> GCVSIIGRLHVNQRGSGSASITAYAQQTRGLLGAIVVSMTGRDRTEQAGEVQILSTVSQSFLGTTISGVLWTVYHGAGNKTLAGLRGPVTQMYSSAEGDLVGWPSPPGTKSLEPCKCGAVDLYLVTRNADVIPARRRGDKRGALLSPRPISTLKGSSGGPVLCPRGHVVGLFRAAVCSRGVAKSIDFIPVETLDVVTRSPTFSDNSTPPAVPQTYQVGYLHAPTGSGKSTKVPVAYAAQGYKVLVLNPSVAATLGFGAYLSKAHGINPNIRT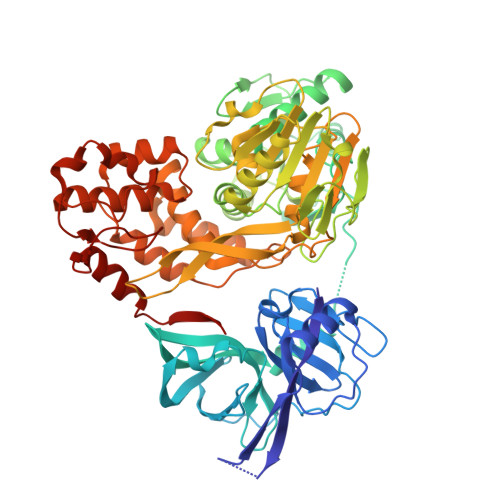GVRTVMTGEAITYSTYGKFLADGGCASGAYDIIICDECHAVDATSILGIGTVLDQAETAGVRLTVLATATPPGSVTTPHPDIEEVGLGREGEIPFYGRAIPLSCIKGGRHLIFCHSKKKCDELAAALRGMGLNAVAYYRGLDVSIIPAQGDVVVVATDALMTGYTGDFDSVIDCNVAVTQAVDFSLDPTFTITTQTVPQDAVSRSQRRGRTGRGRQGTYRYVSTGERASGMFDSVVLCECYDAGAAWYDLTPAETTVRLRAYFNTPGLPVCQDHLEFWEAVFTGLTHIDAHFLSQTKQAGENFAYLVAYQATVCARAKAPPPSWDAMWKCLARLKPTLAGPTPLLYRLGPITNEVTLTHPGTKYIATCMQADLEVMT> MAHHHHHHMSRKRVRAEDIHYWLLKSEPHKFSIDDLAKQKTSPWDGVRNYAARNNMRAMSVGDKVLFYHSNTKEPGVAGLAEVVRLAYDDFTALDK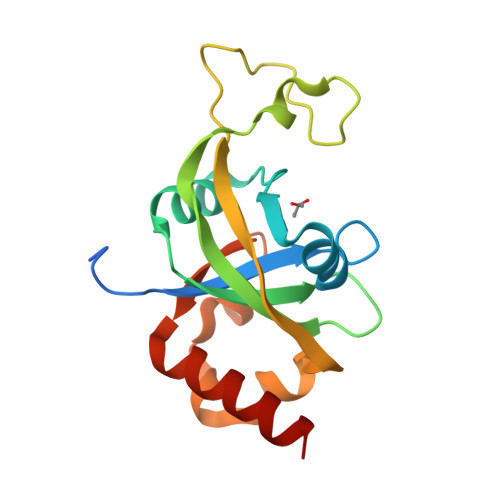TSEYFDPKATKEKNPWKMVDVKFVARWDTVLTLHELKSRRELQKMALFTQRRLSVQPVSASEYAYILRMNEEQQRK>GFGGNDNFG[1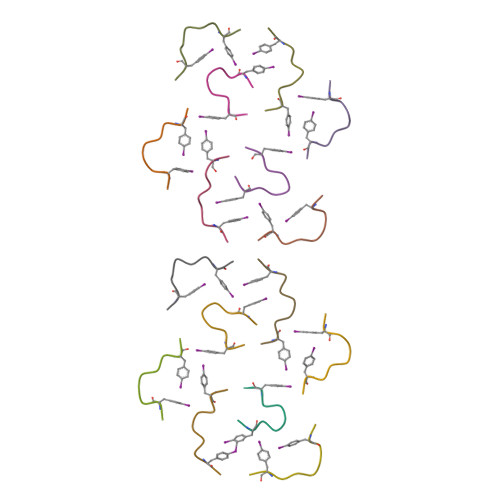6x]> GSNRTLIVTTILEEPYVMYRKSDKPLYGNDRFEGYCLDLLKELSNILGFLYDVKLVPDGKYGAQNDKGEWNGMVKELIDHRADLAVAPLTITYVREKVIDFSK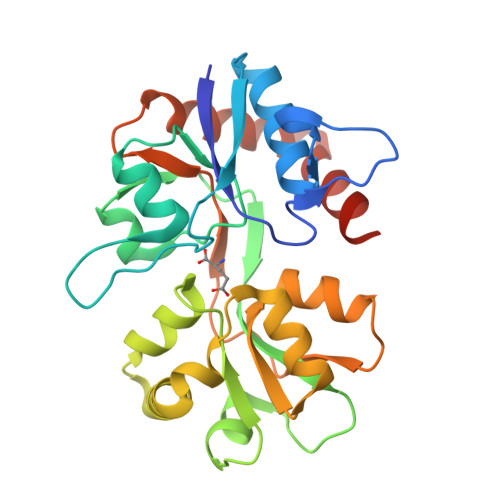PFMTLGISILYRKGTPIDSADDLAKQTKIEYGAVRDGSTMTFFKKSKISTYEKMWAFMSSRQQSALVKNSDEGIQRVLTTDYALLMESTSIEYVTQRNCNLTQIGGLIDSKGYGVGTPIGSPYRDKITIAILQLQEEGKLHMMKEKWWRGNGCPE> MKTPRRRMRLAVFKALFQHEFRRDEDLEQILEEILDETYDKKAKEDARRYIRGIKE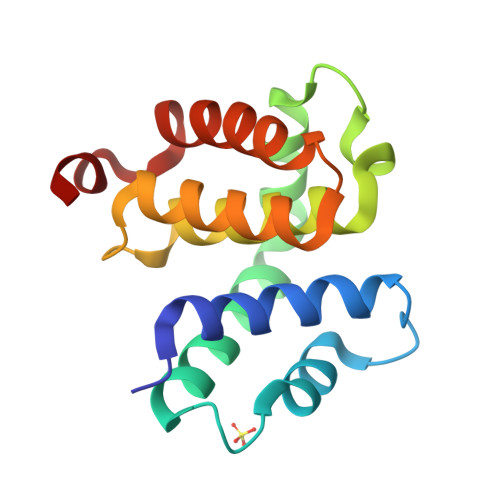NLSMIDDLISRYLEKWSLNRLSVVDRNVLRLATYELLFEKDIPIEVTIDEAIEIAKRYGTENSGKFVNGILDRIAKEHAPKEKFEL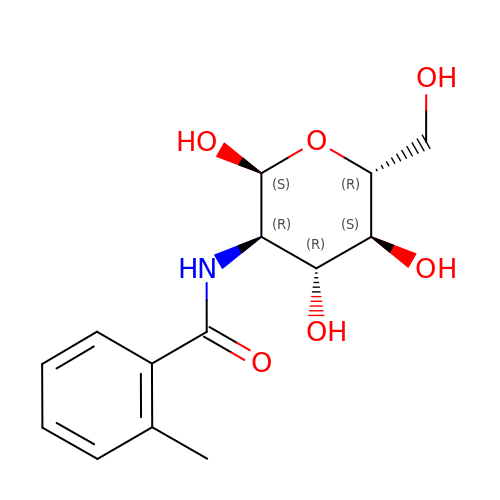2-deoxy-2-{[(2-methylphenyl)carbonyl]amino}-alpha-D-glucopyranose | C14 H19 N O6 | ZWRASUMSHKKCJN-SKENRDBWSA-N>[2x]ISKEYHIDEEVGFALPNPQENLPDFYNDWMFIAKHLPDLIESGQLRERVEKLNMLSIDHLTDHKSQ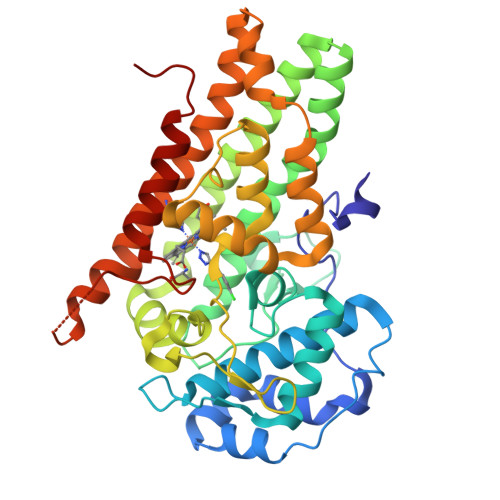RLARLVLGCITMAYVWGKGHGDVRKVLPRNIAVPYCQLSKKLELPPILVYADCVLANWKKKDPNKPLTYENMDVLFSFRDGDCSKGFFLVSLLVEIAAASAIKVIPTVFKAMQMQERDTLLKALLEIASCLEKALQVFHQIHDHVNPKAFFSVLRIYLSGWKGNPQLSDGLVYEGFWEDPKEFAGGSAGQSSVFQCFDVLLGIQQTAGGGHAAQFLQDMRRYMPPAHRNFLCSLESNPSVREFVLSKGDAGLREAYDACVKALVSLRSYHLQIVTKYILIPASQQPKENKTSEDPSKLEAKGTGGTDLMNFLKTVRSTTEKSLLKEG> SMGCVLSLPHRRLVCYCRLFEVPDPNKPQKLGLHQREIFLFNDLLVVTKIFQKKKNSVTYSFRQSFSLYGMQVLLFENQYYPNGIRLTSSVPGADIKVLINFNAPNPQDRKKFTDDLRESIAEVQEMEKH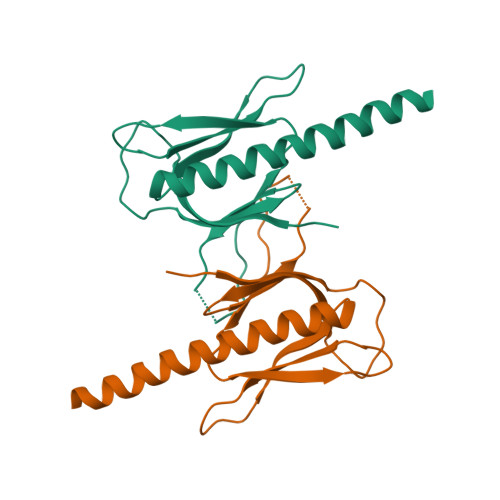RIESELEKQK>[2x]PNFSGNWKIIRSENFEELLKVLGVNVMLRKIAVAAASKPA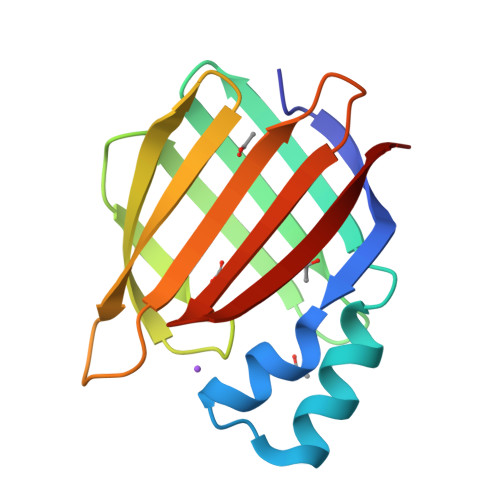VEIKQEGDTFYIKTSTTVRTTEINFKVGEEFEEQTVDGRPCKSLVKWESENKMVCEQKLLKGEGPKTSWTRELTNDGELILTMTADDVVCTRVYVRE>[2x]MAPAEILNGKEISAQIRARLKNQVTQLKEQVPGFTPRLAILQVGNRDDSNLYINVKLKAAEEIGIKATHIKLPRTTTESEVMKYITSLNEDSTVHGFLVQLPLDSENSINTEEVINAIAPEKDVDGLTSINAGRLARGDLNDCFIPCTPKGCLELIKETGVPIAGRHAVVVGRSKIVGAPMHDLLLWNNATVTTCHSKTAHLDEEVNKGDILVVATGQPEMVKG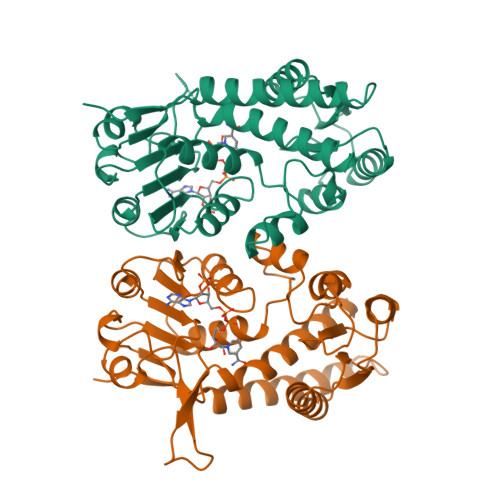EWIKPGAIVIDCGINYVPDDKKPNGRKVVGDVAYDEAKERASFITPVPGGVGPMTVAMLMQSTVESAKRFLEKFKPG>MNLPTAQEVQGLMARYIELVDVGDIEAIVQMXADDATVENPFGQPPIHGREQIAAFYRQGLGGGKVRACLTGPVRASHNGCGAMPFRVEMVWNGQPCALDVIDVMRFDEHGRIQTMQAYWSEVNLSVREPQL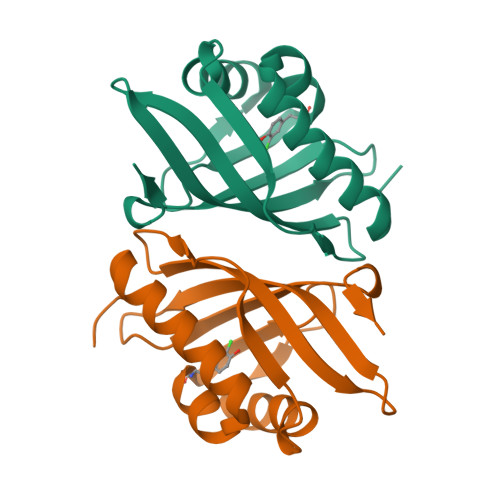VPR[2x]>[2x]C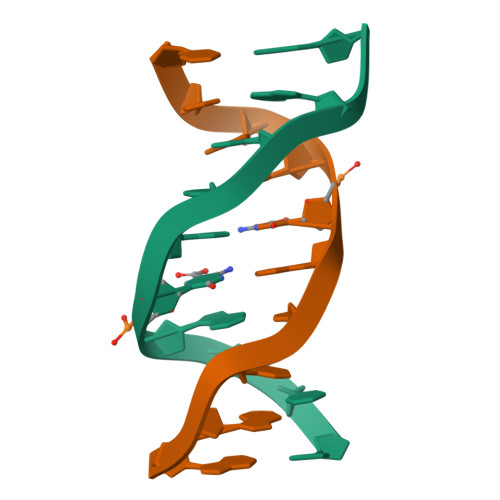CAGXGCTGG> GLVPRGSHMTEVLHIEGHDIKVTNPDKVLFPEDGITKGELVDYYRRISGVMVPLVRGRPMTMQRFPDGIGKEGFFQKEASDYFPDWVHRATLELGKGGIQHQVVCDDAATLVYLASQAMITPHVFLSRIDKVHYPDRLIFDLDPPDNNFETVRSAAKTIREALDAEGYPVYLMTTGSRGLHVVVPLDRSADFDTVRAFARGFGEKLTKKYPDRFTIELSKEKRRGRLFLDYLRNSYGQTGVAPYGVRARSGAPVATPITWDELDDISGSQEYNIRNIMGRMDKRGDAWKYIDKDRTSIKNL

The AP–NHEJ repair complex is primarily composed of a Ku homodimer, DNA ligase (Lig), DNA polymerase (Pol) and a phosphoesterase (PE). Studies on NHEJ repair in Mtu and the archaeon Methanocella paludicola (Mpa) demonstrated that both species possess equivalent core AP–NHEJ components, with orthologous proteins possessing near identical substrate specificities. We discovered that Pol has DNA strand displacement activity during RNA synthesis and that PE resects excessive incorporation to promote efficient break ligation. In this current study, we sought to extend our understanding of AP–NHEJ by comparing crystal structures of the archaeal (Mpa) Pol and PE with those of the established bacterial (M. tuberculosis and P. aeruginosa) DSB repair complexes.

We purified Mpa Pol and crystallized the enzyme, as described in the methods. The structure of Mpa Pol was elucidated at 1.95 Å resolution and a ribbon representation of its structural features is shown in Figure 3A. Mpa Pol shares close structural homology with the bacterial NHEJ polymerases from M. tuberculosis and P. aeruginosa. Based on the close structural similarities between all these polymerases, we can infer that the key structural elements such as Loop 1, Loop 2, the 5′-phosphate binding pocket and the active site perform similar functions in the DSB repair process. Having shown that Mpa Pol is a bona fide member of the AP–NHEJ polymerase family, we next superposed the structure onto that of Mtu PolDom in complex with an incoming nucleotide and DNA. We found that the nucleotide and DNA substrate of the Mtu PolDom structures overlaid precisely with the Mpa Pol structure. The Mpa and Mtu Pols do not have strictly conserved primary amino acid sequences, yet both Loop 1 and Loop 2 adopt similar formations, suggesting a conserved function. We previously reported that Mpa Pol, in common with other NHEJ polymerases, is preferentially a DNA-dependent RNA polymerase with an innate capacity to perform strand displacement synthesis. Examination of the crystal structures of Pol reveals that these enzymes contain a prominent surface protrusion that plays a critical role in this displacement activity. We identify that a conserved arginine residue in this structure acts as a molecular wedge against the annealed interface of the downstream DNA and is critical for enabling displacement synthesis during polymerase extension that occurs during AP–NHEJ repair. The structural architecture of the archaeal NHEJ Pol reported here shows that it is highly similar to the bacterial NHEJ polymerases, supporting conservation in the functional mechanisms of these enzymes in DSB repair.> QNVSLQPPPQQLIVQNKTIDLPAVYQLNGGEEANPHAVKVLKELLSGKQSSKKGMLISIGEKGDKSVRKYSRQIPDHKEGYYLSVNEKEIVLAGNDERGTYYALQTFAQLLKDGKLPEVEIKDYPSVRYRGVVEGFYGTPWSHQARLSQLKFYGKNKMNTYIYGPKDDPYHSAPNWRLPYPDKEAAQLQELVAVANENEVDFVWAIHPGQDIKWNKEDRDLLLAKFEKMYQLGVRSFAVFFDDISGEGTNPQKQAELLNYIDEKFAQVKPDINQLVMCPTEYNKSWSNPNGNYLTTLGD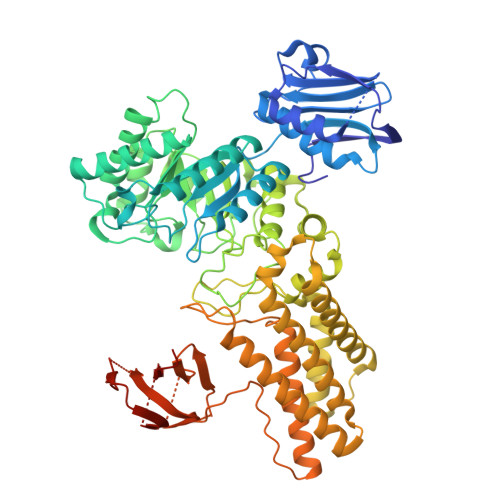KLNPSIQIMWTGDRVISDITRDGISWINERIKRPAYIWWNFPVSDYVRDHLLLGPVYGNDTTIAKEMSGFVTNPMEHAESSKIAIYSVASYAWNPAKYDTWQTWKDAIRTILPSAAEELECFAMHNSDLGPNGHGYRREESMDIQPAAERFLKAFKEGKNYDKADFETLQYTFERMKESADILLMNTENKPLIVEITPWVHQFKLTAEMGEEVLKMVEGRNESYFLRKYNHVKALQQQMFYIDQTSNQNPYQPGVKTATRVIKPLIDRTFATVVKFFNQKFNAHLDATTDYMPHKMISNVEQIKNLPLQVKANRVLISPANEVVKWAAGNSVEIELDAIYPGENIQINFGKDAPCTWGRLEISTDAKEWKTVDLKQKESRLSAGLQKAPVKFVRFTNVSDEEQQVYLRQFVLTIEKK>[3x]KNEPVLDIDGEELRAGEQYYVVSAIWGPGGGGLAL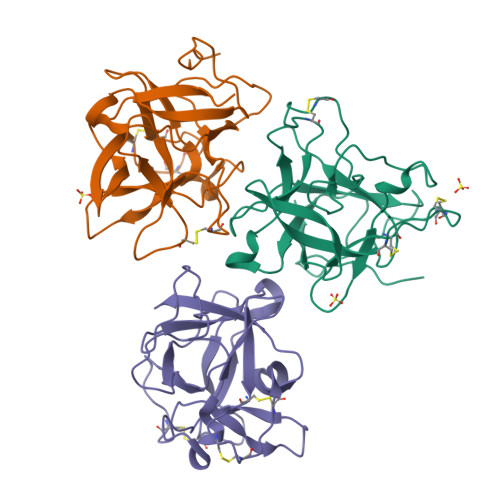GRLTDQKCPEIVVQRRSDSDYGTPVIFHNLDTKDDIVRLSTDFNVEFVPIRDRLCLTSTVWKIDDYDTSTGQWWVTTNGVIGNPGPQTLQSWFKIESGNLGYKFNFCPSVCESCITLCSDIGRYGNDGQMRLALAESGWPFVFKKASSNIKQVVNAKH>SELDAKLNKLGVDRIAISPYKQWTRGYM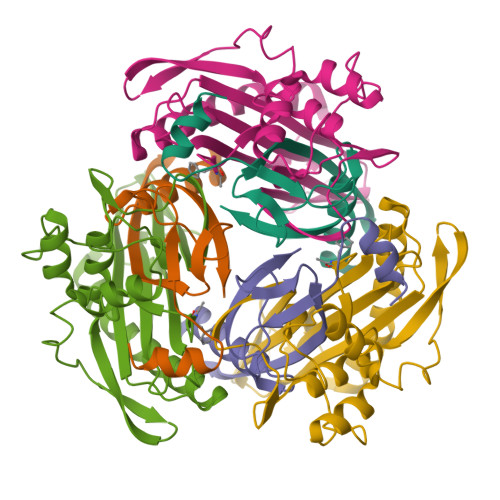EPGNIGNGYVTGLKVDAGVRDKSDDDVLDGIVSYDRAETKNAYIGQINMTTAS[3x];>[3x]XFTGVQGRVIGYDILRSPEVDKAKPLFTETQWDGSELPIYDAKPLQDALVEYFGTEQDRRHYPAPGSFIVCANKGVTAERPKNDADMKPGQGYGVWSAIAISFAKDPTKDSSMFVEDAGVWETPNEDELLEYLEGRRKAMAKSIAECGQDAHASFESSWIGFAYTMMEPGQIGNAITVAPYVSLPIDSIPGGSILTPDKDMEIMENLTMPEWLEKMGYKSLSANNALKY5-{2-[(1R)-2-{(carboxymethyl)[(thiophen-2-yl)methyl]amino}-2-oxo-1-{[(2-oxo-1,2-dihydroquinolin-6-yl)sulfonyl]amino}ethyl]phenoxy}pentanoic acid | 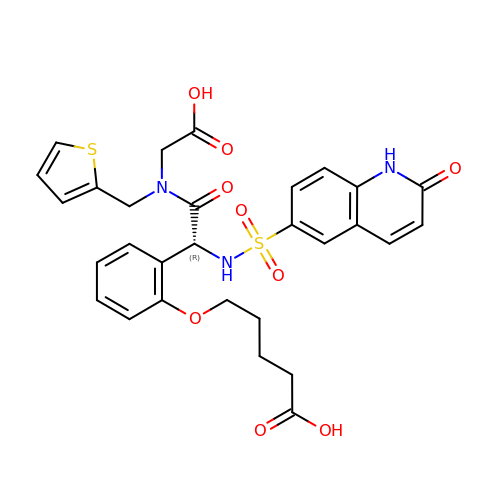C29 H29 N3 O9 S2 | VMCJXXUCJJAXMA-MUUNZHRXSA-N>[2x]MGSDKIHHHHHHENLYFQGMKFAVAVSGDRVNGPGESEEVQIYETDGGNVRLIEKYSNPALNATAARGVFMLKSALDHGANALVLSEIGSPGFNFIKNKMD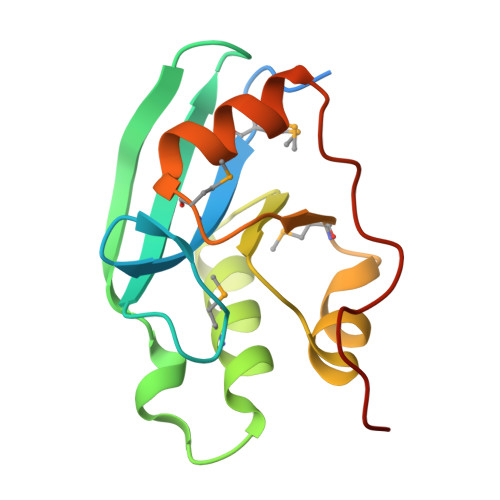VYIVPEMPVADALKLILEGKVSPATAPTHDHGHHH>MRIAVIGGGSSYTPELVKGLLDISEDVRIDEVIFYDIDEEKQKIVVDFVKRLVKDRFKVLISDTFEGAVVDAKYVIFQFRPGGLKGRENDEGIPLKYGLIGQETTGVGGFSAALRAFPIVEEYVDTVRKTSNATIVNFTNPSGHITEFVRNYLEYEKFIGLCNVPINFIREIAEMFSARLEDVFLKYYGLNHLSFIEKVFVKGEDVTEKVFENLKLKLSNIPDEDFPTWFYDSVRLIVNPYLRYYLMEKKMFKKISTHELRAREVMKIEKELFEKYRTAVEIPEELTKRGGSMYSTAAAHLIRDLETDEGKIHIVNTRNNGSIENLPDDYVLEIPCYVRSGRVHTL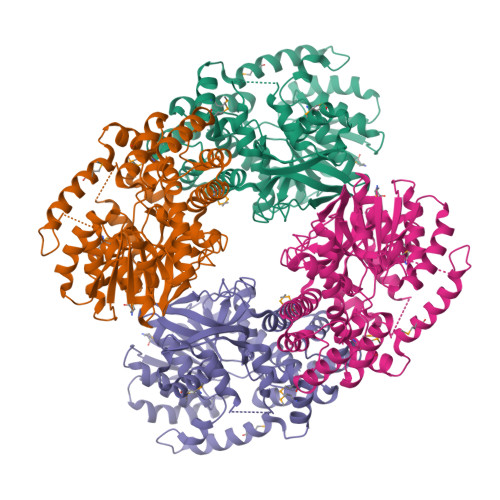SQGKGDHFALSFIHAVKMYERLTIEAYLKRSKKLALKALLSHPLGPDVEDAKDLLEEILEANREYVKLG[8x]> VQSDTHIFIIMGASGDLAKKKIYPTIWWLFRDGLLPENTFIVGYARSRLTVADIRKQSEPFFKATPEEKLKLEDFFARNSYVAGQYDDAASYQRLNSHMNALHLGSQANRLFYLALPPTVYEAVTKNIHESCMSQIGWNRIIVEKPFGRDLQSSDRLSNHISSLFREDQIYRIDHYLGKEMVQNLMVLRFANRIFGPIWNRDNIACVILTFKEPFGTEGRGGYFDEFGIIRDVMQNHLLQMLCLVAMEKPASTNSDDVRDEKVKVLKCISEVQANNVVLGQYVGNPDGEGEATKGYLDDPTVPRGSTTATFAAVVLYVENERWDGVPFILRCGKALNERKAEVRLQFHDVAGDIFHQQCKRNELVIRVQPNEAVYTKMMTKKPGMFFNPEESELDLTYGNRYKNVKLPDAYERLILDVFCGSQMHFVRSDELREAWRIFTPLLHQIELEKPKPIPYIYGSRGPTEADELMKRVGFQYE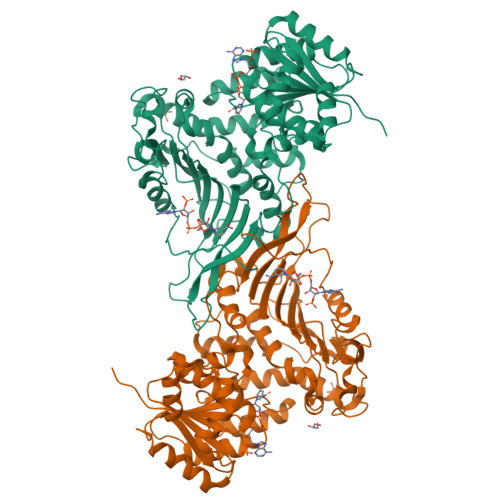GTYKWVNPHKL>[2x]MADTQYILPNDIGVSSLDCREAFRLLSPTERLYAYHLSRAAWYGGLAVLLQTSPEAPYIYALLSRLFRAQDPDQLRQHALAEGLTEEEYQAFLVYAAGVYSNMGNYKSFGDTKFVPNLPKEKLERVILGSEAAQQHPEEVRGLWQTCGELMFSLEPRLRHLGLGKEGITTY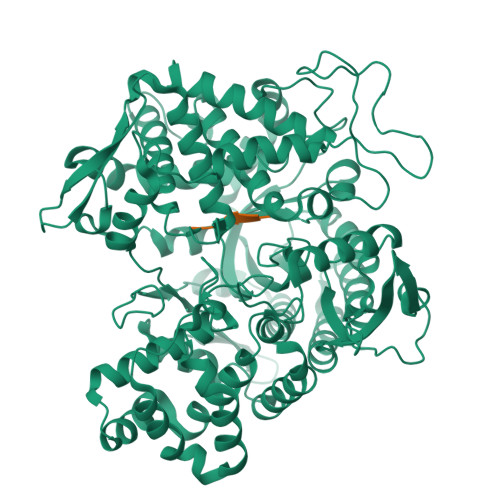FSGNCTMEDAKLAQDFLDSQNLSAYNTRLFKEVDGEGKPYYEVRLASVLGSEPSLDSEVTSKLKSYEFRGSPFQVTRGDYAPILQKVVEQLEKAKAYAANSHQGQMLAQYIESFTQGSIEAHKRGSRFWIQDKGPIVESYIGFIESYRDPFGSRGEFEGFVAVVNKAMSAKFERLVASAEQLLKELPWPPTFEKDKFLTPDFTSLDVLTFAGSGIPAGINIPNYDDLRQTEGFKNVSLGNVLAVAYATQREKLTFLEEDDKDLYILWKGPSFDVQVGLHALLGHGSGKLFVQDEKGAFNFDQETVINPETGEQIQSWYRSGETWDSKFSTIASSYEECRAESVGLYLCLHPQVLEIFGFEGADAEDVIYVNWLNMVRAGLLALEFYTPEAFNWRQAHMQARFVILRVLLEAGEGLVTITPTTGSDGRPDARVRLDRSKIRSVGKPALERFLRRLQVLKSTGDVAGGRALYEGYATVTDAPPECFLTLRDTVLLRKESRKLIVQPNTRLEGSDVQLLEYEASAAGLIRSFSERFPEDGPELEEILTQLATADARFW;>VVYPW[2x]>[2x]MHHHHHHDYKDDDDKAPVQAADEMYDSNPHPDRRQLVSNGFEVNLPDQVEVIVRDLPDPSKVKEERTRLMGYWFVHWFDGKLFHLRIKAGGPNVDGEHRAIRTAEHPWLLRARLDDALEEALPKYAAVKKRPFTFLAQKDELIDAAATAAGLSHRLLNSFKVIPRFALSPKIYEPVDGTTRVGVFVTIGMRYDIEASLRDLLEAGIDLRGMYVVRRKRQPGERGLLGRVRAISDDMVQLFEETDLASVNVND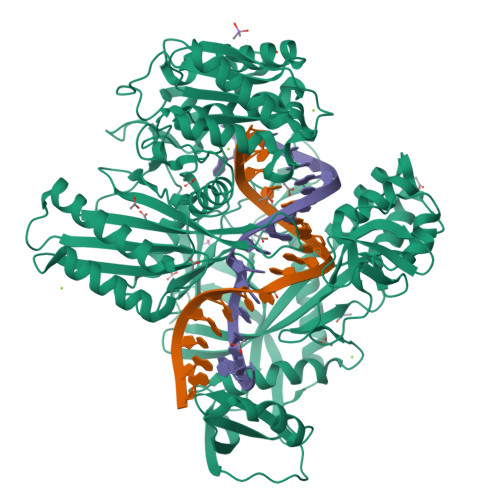AKLEGSKENFTRCLSALLGHNYKKLLNALDDQEAGYRTGPRFDDAVRRMGEFLAKKPIRLADNINAQVGDRIVFSNEGQARNVRLAPKVEYVFDRTGAKSAEYAWRGLSQFGPFDRPSFANRSPRILVVYPSSTQGKVENFLSAFRDGMGSNYSGFSKGFVDLMGLTKVEFVMCPVEVSSADRNGAHTKYNSAIEDKLAGAGEVHAGIVVLFEDHARLPDDRNPYIHTKSLLLTLGVPTQQVRMPTVLLEPKSLQYTLQNFSIATYAKLNGTPWTVNHDKAINDELVVGMGLAELSGSRTEKRQRFVGITTVFAGDGSYLLGNVSKECEYEGYSDAIRESMTGILRELKKRNNWRPGDTVRVVFHAHRPLKRVDVASIVFECTREIGSDQNIQMAFVTVSHDHPFVLIDRSERGLEAYKGSTARKGVFAPPRGAISRVGRLTRLLAVNSPQLIKRANTPLPTPLLVSLHPDSTFKDVDYLAEQALKFTSLSWRSTLPAATPVTIFYSERIAELLGRLKSIPNWSSANLNIKLKWSRWFL> ANSMIRLNVFVRVNETNREKAIEAAKELTACSLKEEGCIAYDTFESSTRRDVFMICETWQNAEVLAAHEKTAHFAQYVGIIQELAEM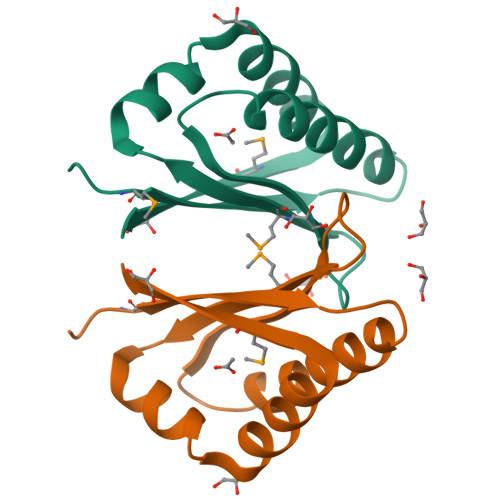KLEKFEF>[2x]SNANYMETGDQRFGDLVFRQLAPNVWQHTSYLDMPGFGAVASNGLIVRDGGRVLVVDTAWTDDQTAQILNWIKQEINLPVALAVVTHAHQDKMGGMDALHAAGIATYANALSNQLAPQEGMVAAQHSLTFAANGWVEPATAPNFGPLKVFYPGPGHTSDNITVGIDGTDIAFGGCLIKDSKAKSLGNLGDADTEHYAASARAFGAAFPKASMIVMSHSAPDSRAAITHTARMADKLR

NDM-1 has been reported to be a highly potent carbapenem-hydrolyzing, zinc-dependent MBL. NDM-1 is an extended spectrum zinc dependent β-lactamase capable of hydrolyzing nearly all classes of β-lactams, impairing the ability to treat life-threatening infections with intravenously and orally available carbapenems.. NDM-1 resembles the common β-lactamase fold, although it shows low sequence similarity to β-lactamases deposited in PDB (20–33% sequence identity). Our results show that NDM-1 is unique among other MBLs due to its enlarged and flexible active site, and explain the observed extended spectrum β-lactamase activity.

Three of our apoNDM-1 structures are zinc-free and are the first structures of a wild-type apo-enzyme in subclass B1. No zinc is found in the structure and only an acetate ion can be modeled in the active site interacting with His250. The three apoNDM-1 structures include two pairs of monomers A and B and one monomer A, and the structure of monometalated NDM-1 (mZnNDM-1 Δ36NY) includes four monomers (A, B, C, D), respectively in the asymmetric unit, providing nine crystallographically independent views of the molecule for NDM-1 Δ38, NDM-1 Δ36NY (monoclinic), NDM-1 Δ36NY (orthorhombic), mZn-NDM-1 Δ36NY (tetragonal). In our three apo and one monozinc structures, there are nine independent representations of NDM-1 molecules with different crystallization conditions and packing environments. In these structures, most active site loops show very small conformational changes with the exception of ASL1 and to some extent ASL4. These are key loops contributing to the expansion of active site accessibility. In apoNDM-1 structure conformations of some of these residues are very similar to zinc-bound states (His120, Asp124, and His250), while others show somewhat different side chain orientations (His122, His189, and Cys208). Cys208 exists in two orientations in apo-state, one is similar to the zinc bound state and the other is rotated about 45 and 90 degrees in chain A and B, respectively.> TGGVQTVTLIPGDGIGPEISAAVMKIFDAAKAPIQWEERNVTAIQGPGGKWMIPSEAKESMDKNKMGLKGPLKTPIAAGHPSMNLLLRKTFDLYANVRPCVSIEGYKTPYTDVNIVTIRENTEGEYSGIEHVIVDGVVQSIKLITEGASKRIAEFAFEYARNNHRSNVTAVHKANIMRMSDGLFLQKCREVAESCKDIKFNEMYLDTVCLNMVQDPSQFDVLVMPNLYGDILSDLCAGLIGGLGVTPSGNIGANGVAIFESVHGTAPDIAGKDMANPTALLLSAVMMLRHMGLFDHAARIEAACFATIKDGKSLTKDLGGNAKCSDFTEEICRRVKDLD;> FSEQTIPPSAKYGGRHTVTMIPGDGIGPELMLHVKSVFRHACVPVDFEEVHVSSNADEEDIRNAIMAIRRNRVALKGNIETNHNLPPSHKSRNNILRTSLDLYANVIHCKSLPGVVTRHKDIDILIVRENTEGEYSSLEHESVAGVVESLKIITKAKSLRIAEYAFKLAQESGRKKVTAVHKANIMKLGDGLFLQCCREVAARYPQITFENMIVDNTTMQLVSRPQQFDVMVMPNLYGNIVNNVCAGLVGGPGLVAGANYGHVYAVFETATRNTGKSIANKNIANPTATLLASCMMLDHLKLHSYATSI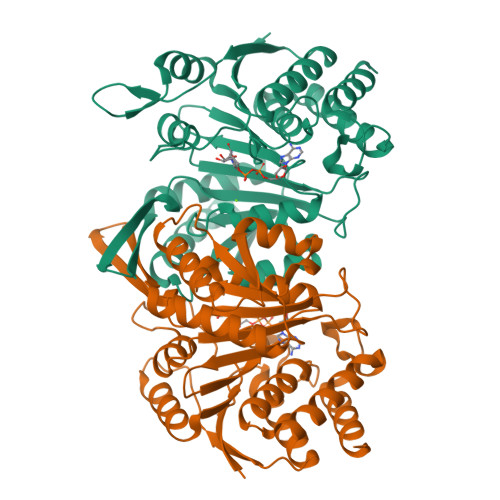RKAVLASMDNENMHTPDIGGQGTTSEAIQDVIRHIRVINGRAVEA> MVAKGRIIRVTGPLVVADGMKGAKMYEVVRVGELGLIGEIIRLEGDKAVIQVYEETAGVRPGEPVVGTGASLSVELGPRLLTSIYDGIQRPLEVIREKTGDFIARGVTAPALPRDKKWHFIPKAKVGDKVVGGDIIGEVPETSIIVHKIMVPPGIEGEIVEIAEEGDYTIEEVIAKVKTPSGEIKELKMYQRWPVRVKRPYKEKLPPEVPLITGQRVIDTFFPQAKGGTAAIPGPFGAGKTVTQHQLAKWSDAQVVIYIGCGERGNEMTDVLEEFPKLKDPKTGKPLMERTVLIANTSNMPVAAREASIYTGITIAEYFRDMGYDVALMADSTSRWAEALREISGRLEEMPGEEGYPAYLASKLAEFYERAGRVVTLGSDYRVGSVSVIGAVSPPGGDFSEPVVQNTLRVVKVFWALDADLARRRHFPAINWLTSYSLYVDAVKDWWHKNIDPEWKAMRDKAMALLQKESELQEIVRIVGPDALPERERAILLVARMLREDYLQQDAFDEVDTYCPPEKQVTMMRVLLNFYDKTME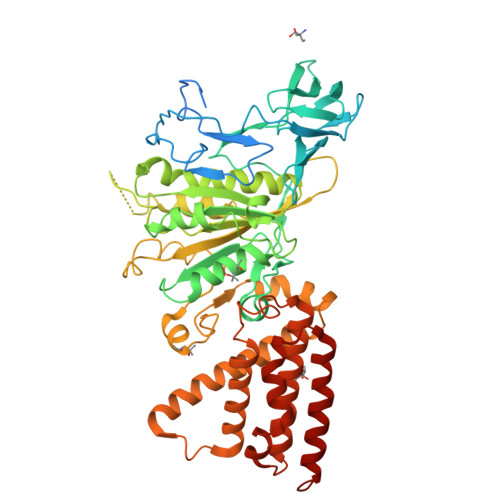AINRGVPLEEIAKLPVREEIGRMKFERDVSKIRSLIDKTNEQFEELFKKYGA2-chloro-4-hydroxy-3-(2'-hydroxybiphenyl-4-yl)-6-oxo-6,7-dihydrothieno[2,3-b]pyridine-5-carbonitrile 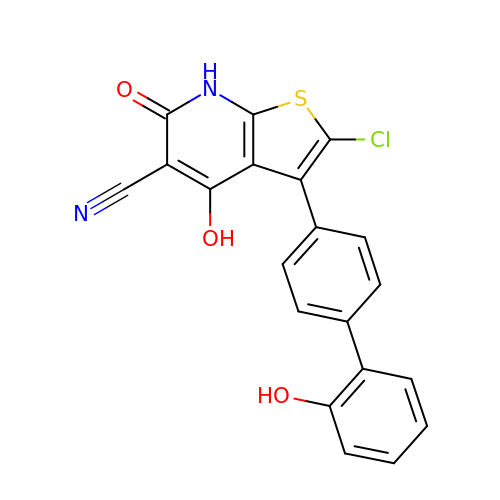| C20 H11 Cl N2 O3 S | JGMADXMPAZATOC-UHFFFAOYSA-N>MIERGKFRSLTLVNWNGFFARTFDLDELVTTLSGGNGAGKSTTMAAFVTALIPDLTLLHFRNTTEAGATSGSRDKGLHGKLRAGVCYSTLDVINSRHQRVVVGVRLQQVAGRDRKVDIKPFMIQGLPTAIQPTQLLTENVGERQARVLPLNELKDRLDEMEGVQFKQFNSITDYHAQMFDLGVIPKRLRSASDRSKFYRLIEASLYGGISSAITRSLRDYLLPENSGVRKAFQDMEAALRENRITLEAIRVTQSDRDLFKHLITEATSYVSADYMRHANERRTHLDEALALRGELFGSHKQLATEQYRHVEMARELAEQSGASSDLETDHQAASDHLNLVQTAMRQQEKIDRYQVDLEELSYRLEEQTDVVEEAGELQAEYEARTEATEQEVDELKSQLADYQQALDVQQTRAIQYQQALQALERARELCRLPDLSVDNAEEWLETFQAKEQQATEALLALEQKLSVADAAHNQFEQAYQLVKNIVGETSRSEAWQSARELLRDWPSQRHLADRVQPLRMRLSELEQRLNNQQNAERLLSEFCKRQGRQYQAEDLEALQNELEARQEALSLSVNEGGERRMEMRQELEQLKQKIQSLTARAPVWLAAQDTLNQLCEQSGETLASSNDVTEYMQQLLEREREATVERDEVAAQKRELEKQIERLSQPSGAEDSRMIALAERFGGVLLSEIYDDITIDDAPYFSALYGPARHGIVVPDLSLVRPHLETLEDCPEDLYLIEGDPQSFDDSVFNAEEQTNAVLVKSSDRQWRYSRYPELPLFGRAARENRLEALNLERDALAERYATLSFDVQKIQRAHQAFSQFVGKHLSVAFDTDPEAEIRELRQRHTELEREVSRFEDQTQQQRQQYAQAKESLTTLNRLIPQVTLLLDETLIDRVEEVREEMDEAQEAARFLQQHGSALTKLEPMVAVLQSDPQQHEQLQQDYETAKHSQHQAKQQAFALVEIVQRRVHFSYSDSAGMLSENADLNDKLRQRLEHAESDRSRAREQLRQQQAQYSQFNQVLASLKSSYETKQDMLKELLQEMKDIGVQADANAEMRARERRDRLHEALSVNRSRVNQLEKQIAFCEAEMENVQKKLRKLERDYYQIREQVVSAKAGWCAVMRMVKDNGVERRLHRRELAYMEGGALRSMSDKALGALRLAVADNEHLRDALRLSEDPKRPERKVQFFIAVYQHLRERIRQDIIRTDDPVDAIEQMEIELARLTEELTAREQKLAISSKSVANIIRKTIQREQNRIRMLNQGLQAVSFGQVRGVRLNVNVRESHAILLDVLSEQQEQHQDLFNSQRLTFSEAMAKLYQRLNPQVDMGQRLPQTIGEELLDYRNYLELDVEVNRGSDGWLKAESGALSTGEAIGTGMSILVMVVQSWEEESRRLRGKDISPCRLLFLDEAARLDAKSIATLFELCERLQMQLIIAAPENISPEKGTTYKLVRKVFKNHEHVHVVGLRGFGQDAPATQLISDVTA[2x];>[2x]MSEYSQTVPELVSWARKNDFSISLPVERLAFLMAIAVLNSERLDGEMSEGELIDAFREVCKGFEQTAESVAVRANNAINDMVRQKLLNRFTSELADGNAIYRLTPLGISISDYYIRQREFSTLRLSMQLSIVANELHRAAEAAEEGGDEFHWHRNVFAPLKYSVAEIFDSIDMSQRLMDEQQNFVKEDIAALLNQDWQAAIANCEQLLSETSGTLRELQDTLEAAGDKLQANLLRIQDANMGSGGSELVDKLVFDLQSKLDRIISWGQQAIDLWIGYDRHVHKFIRTAIDMDKNRIFSQRLRQSVQHYFDNPWTLTVANAERLLDMRDEELALRNEEVTGELPLELEYEEFSEINDQLAAMIEKALLVYQQEQRPLDLGAVLRDYLAQHPLPRHFDVARILVDQAVRLGVAEADFSGLPAEWLAINDYGAKVQAHVIDTY;>MSSTHIEQFMPVKLAQALANSLFPELDSQLRAGRHIGIDDLDNHAFLMDFQEQLEEFYARYNVELIRAPEGFFYLRPRSTTLIPRSVLSELDMMVGKILCYLYLSPERLANQGIFTSQELYEELISLADEGKLMKFVNQRSSGSDLDKQKLQEKVRTTLNRLRRLGMVYFLPNNNNKFTITEAVFRFGADVRSGDDPREIQLRMIRDGEAMPVEGSLSLDDSENDETPDNSAEGAGDEQP[3x];>[2x]MSTIEERVKKIIGEQLGVKQEEVTNNASFVEDLGADXLDTVELVMALEEEFDTEIPDEEAEKITTVQAAIDYINGHQA

MukBEF folds the chromosome of Escherichia coli and related bacteria. The SMC protein MukB dimerizes at its ‘‘hinge’’ domain, which connects via the long coiled-coil ‘‘arm’’ to the ABC-type ATPase ‘‘head’’ domain. The heads are bridged by the kleisin MukF, whereby the C-terminal winged-helix domain (cWHD) of MukF binds the ‘‘cap’’ surface of one MukB, and the N-terminal middle domain (MD) binds the coiled-coil ‘‘neck’’ of the other MukB. MukF also recruits the dimeric KITE protein MukE.

Focused sub-classification of the particle images revealed a DNA-bound structure. The DNA was captured directly at the open gate, while the proteins adopted a conformation virtually identical to the open-gate state. DNA-binding surfaces were largely contributed by MukE and MukF, and to a lesser extent by the root of the ν-MukB neck. Compared with the apo state, MukE and MukF had aligned their DNA-binding surfaces to enable DNA capture. The DNA was not entrapped inside the complex but bound at its periphery without contacting the top surface of the heads. MukE employed a DNA-binding mode overall similar to its role in DNA clamping; however, the DNA followed a differently bent path along its surface. As the captured DNA is positioned at the open neck gate but not entrapped, we reason that entrapment may be achieved by ingestion through the gate. We propose that the DNA-bound structure obtained here represents this capture state. The capture state, however, requires ATP binding only but not hydrolysis and can thus occur before DNA entrapment. While ATP binding exposes the DNA capture site, ATP hydrolysis triggers closing of the neck gate and ingestion of the captured DNA.>[2x]GPSRGAQNSISWEVQRFDGWYNNLMEHRWGSKGSRLQRLV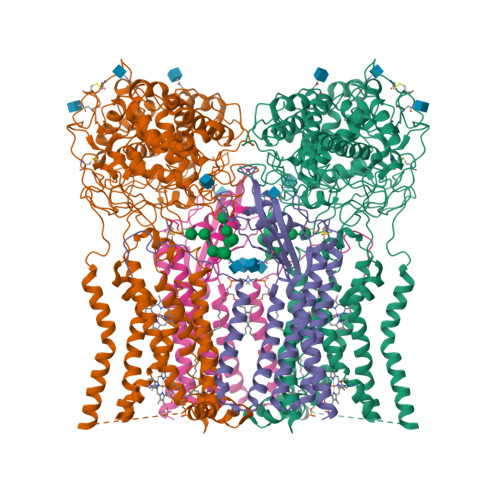PASYADGVYQPLKEPYLPNPRHLSNRVMRGSAGQPSLRNRTVLGVFFGYHVLSDLVSVETPGCPAEFLNIYIPHGDPVFDPDKRGNVVLPFQRSRWDRNTGQSPSNPRDQSNQVTGWLDGSAIYGSSHSWSDTLRSFSGGQLASGPDPAFPSDSQSSLLMWMAPDPSTGQGGPRGVYAFGAQRGNREPFLQALGLLWFRYHNLCARKLAQEHPHWGDEELFQHARKRVIATYQNIAMYEWLPSFLKQTPPEYPGYRPFLDPSISPEFVVASEQFLSTMVPSGVYMRNASCHFQGIPSHNSSVSGALRVCNSYWSREHPKLQRAEDVDALLLGMASQIAEREDHVVVEDMQDFWPGPLKFSRTDYLASCLQRGRDLGLPSYTKAREALGLSPISHWQDINPALSRSNGTVLEATAALYNQDLSRLELLPGGLLESHGDPGPLFSTIVLDQFVRLRDGDRYWFENTRNGLFSKEEIAEIRNTSLRDILVAVTNVDPSALQPNVFFWLAGDPCPQPSQLSAKGLPACAPLFIRDYFEGSGFGFGLTIGTLCCFPLVSLLSAWIVARLRKRNFKRLQRQDRQSIMSEKLVGGVEALEWQGRNEPCRPVLVHLQPGQIRVVDGRLTVLRTIQLRPPQQVNLILSSNRGRRTLLLKIPKEYDLVLLFNMEEERQALVENVRGALKENGLSFQEWELREQELMRAAVTRQQRGHLLETFFRHLFSQVLDINQADAGTLPLDSSTKVREALTCELSRAEFADSLGLKPQDMFVESMFSLADKDGNGYLSFREFLDILVVFMKGSPEEKSRLMFRMYDFDGNGLISKDEFIRMLRSFIEISNNCLSKAQLAEVVESMFRESGFQDKEELTWEDFHFMLRDHDSDLRFTQLCVKGVEVPEVIKNLCRRASYISQEKICPSPRMSAHCARNNMKTASSPQRLQCPMDTDPPQEIRRRFGKKVTSFQPLLFTEAHREKFQRSRRHQTVQQFKRFIENYRRHIGCVAVFYTITGALFLERAYYYAFAAHHSGITDTTRVGIILSRGTAASISFMFSYILLTMCRNLITFLRETFLNRYIPFDAAVDFHRLIASTAIILTVLHSAGHVVNVYLFSISPLSVLSCLFPGLFHDDGSEFPQKYYWWFFQTVPGLTGVLLLLALAIMYVFASHHFRRRSFRGFWLTHHLYIFLYILLIIHGSFALIQMPRFHIFFLVPAIIYVGDKLVSLSRKKVEISVVKAELLPSGVTHLRFQRPQGFEYKSGQWVRIACLALGTTEYHPFTLTSAPHEDTLSLHIRAAGPWTTRLREIYSPPTGDTCARYPKLYLDGPFGEGHQEWHKFEVSVLVGGGIGVTPFASILKDLVFKSSVSCQVFCKKIYFIWVTRTQRQFEWLADIIREVEENDRQDLVSVHIYITQLAEKFDLRTTMLYICERHFQKVLNRSLFTGLRSITHFGRPPFEPFFNSLQEVHPQVRKIGVFSCGPPGMTKNVEKACQLINRQDRTHFSHHYENF;>MAALGHTLPFYTGTKPTFPMDTTLAVIITIFLTALVTFIIILPGIRGKTRLFWLLRVVTSLFIGAVILAVNFSSEWSVGHVNANTTYKAFSPKWVSVDVGLQIGLGGVNITLTGTPVQQLNETINYNEAFAWRLGRSYAEEYAKALEKGLPDPVLYLAEKFTPRSPCGLYNQYRLAGHYASAMLWVAFLCWLLANVMLSMPVLVYGGHMLLATGLFQLLALFFFSMTTSLISPCPLRLGTAVLHTHHGPAFWITLATGLLCILLGLVMAVAHRMQPHRLKAFFNQSSEDPVLEWGSEEGGLLSPHYRSIAESPETQDIPMSVASSETCFKEEHPKESDCSL[2x]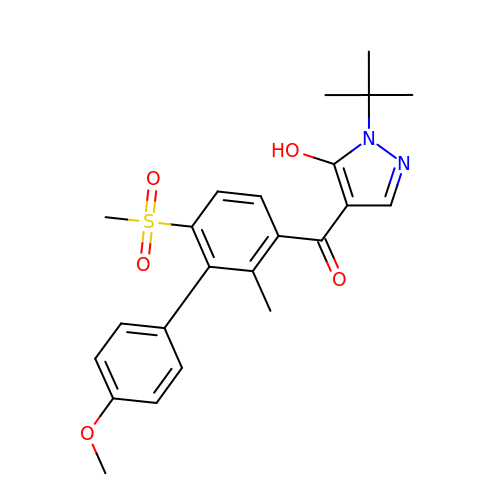(1-TERT-BUTYL-5-HYDROXY-1H-PYRAZOL-4-YL)[6-(METHYLSULFONYL)-4'-METHOXY-2-METHYL-1,1'-BIPHENYL-3-YL]METHANONE | C23 H26 N2 O5 S | AVFXBZIGDFPGBY-UHFFFAOYSA-N7-cyclopentyl-N,N-dimethyl-2-{[5-(piperazin-1-yl)pyridin-2-yl]amino}-7H-pyrrolo[2,3-d]pyrimidine-6-carboxamide 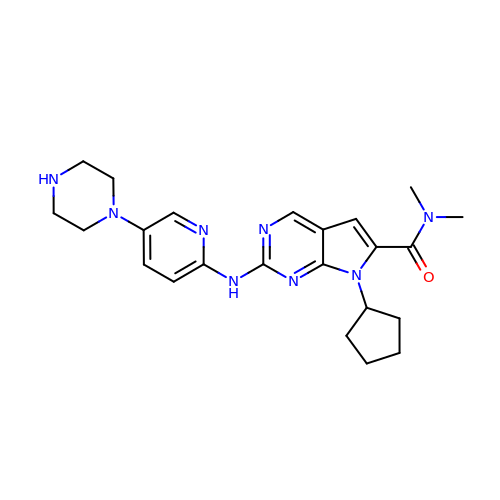| C23 H30 N8 O | RHXHGRAEPCAFML-UHFFFAOYSA-N> GHMAENREPRGAVEAELDPVEYTLRKRLPSRLPRRPNDIYVN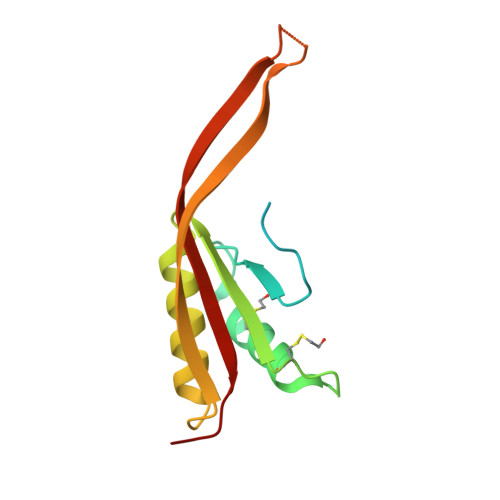MKTDFKAQLARCQKLLDGGARGQNACSEIYIHGLGLAINRAINIALQLQAGSFGSLQVAANTSTVELVDELEPETDTREPLTRIRNNSAIHIRVFRVTPK> SSLSPTEGKGSGLQGHIIENPQYFSDACVHHIKRRDIVLKWELGEGAFGKVFLAECHNLLPEQDKMLVAVKALKEASESARQDFQREAELLTMLQHQHIVRFFGVCTEGRPLLMVFEYMRHGDLNRFLRSHGPDAKLLAGGEDVAPGPLGLGQLLAVASQVAAGMVYLAGLHFVHRDLATRNCLVGQGLVVKIGDFGMSRDIYSTDYYRVGGRTMLPIRWMPPESILYRKFTTESDVWSFGVVLWEIFTYGKQPWYQLSNTEAIDCITQGRELERPRACPPEVYAIMRGCWQREPQQRHSIKDVHARLQALAQAPPVYLDVLGHH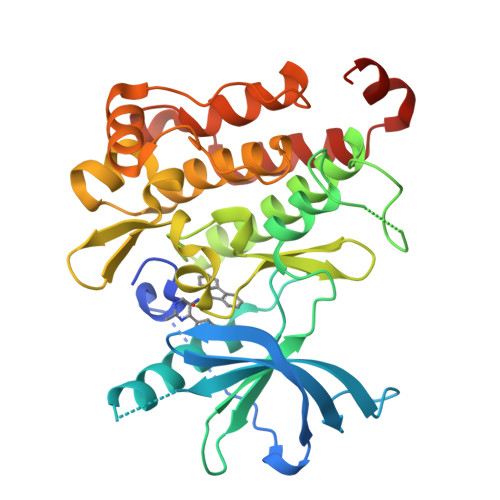HHHH>[2x]MTKAVPDKFQGFAVSDPKNWNRPKLASYERKQINPHDVVLKNEVCGLCYSDIHTLSAG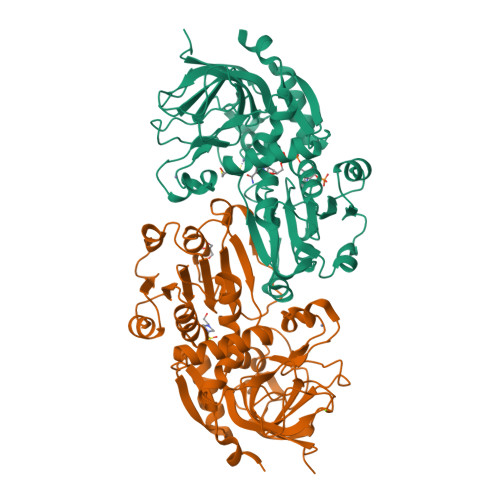WQPLQRDNLVVGHEIIGEVIAVGDEVTEFKVGDRVGIGAASSSCRSCQRCDSDNEQYCKQGAATYNSKDVRSNNYVTQGGYSSHSIADEKFVFAIPEDLPSSYGAPLMCAGITVFSPLIRNLGLDARGKNVGIIGIGGLGHLALQFANAMGANVTAFSRSSSKKEQAMKLGAHDFVATGEDKTWYKNYDDHFDFILNCASGIDGLNLSEYLSTLKVDKKFVSVGLPPSEDKFEVSPFTFLQQGASFGSSLLGSKTEVKEMLNLAAKHNVRPMIEEVPISEENCAKALDRCHAGDVRYRFVFTDFDKAFA> GAHMSIDETVARYKAQFTQLDTMMSKLNNTSSYLTQQFTAMNKSGGSGGSGSGGSGGMTSTVEFINRWQRIALLSQSLLELAQRGEWDLLLQQEVSYLQSIETVMEKQTPPGITRSIQDMVAGYIKQTLDNEQLLKGLLQQRLD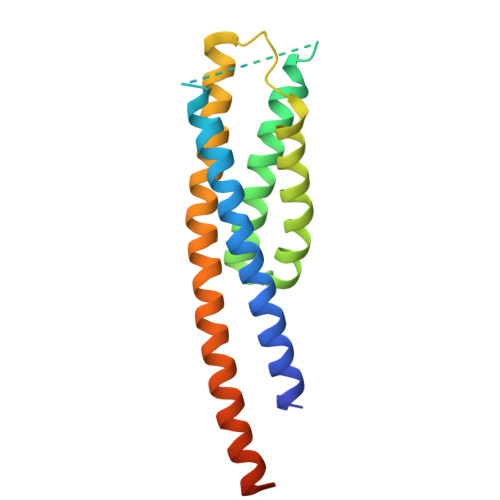ELSSLIGQSTRQKSLNNAYGRLSGMLLVPDAPGAS>VPSPYLLSDKEVREIVQQSLSVGNFAARLLVRLFPELFTTENLRLQYNHSGACNKKQLDPTRLRLIRHYVEAVYPVEKMEEVWHYECIPSIDERC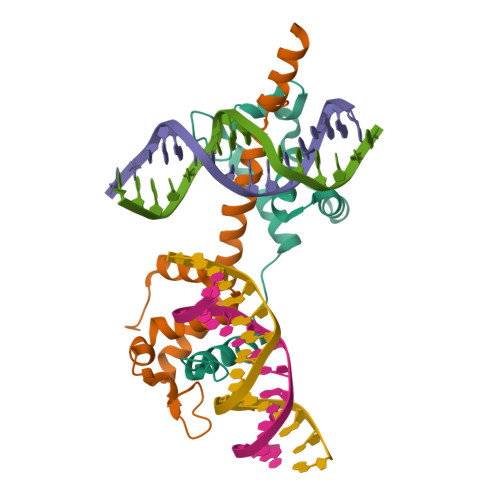RRPNRKKCDILKKAKKVEK[4x]>MSEFNITETYLRFLEEDTEMTMPIAAIEALVTLLRIKTPETAAEMINTIKSSTEELIKSIPNSVSLRAGCDIFMRFVLRNLHLYGDWENCKQHLIENGQLFVSRAKKSRNKIAEIGVDFIADDDIILVHGYSRAVFSLLNHAANKFIRFRCVVTESRPSKQGNQLYTLLEQKGIPVTLIVDSAVGAVIDKVDKVFVGAEGVAESGGIINLVGTYSVGVLAHNARKPFYVVTESHKFVRMFPLSSDDLPMAGPPLDFTRRTDDLEDALRGPTIDYTAQEYITALITDLGVLTPSAVSEELIKMWYD[2x];>MSESEAKSRSATPPSKAKQATPTTTAAANGEKKLTNKELKELKKQEKAAKRAAMKQANGISIEQQQQQAQMKKEKKQLQREQQQKREQKQKNANKKKQNERNVKKSTLFGHLETTEERRATILALTSAVSSPKTSRITAAGLMVPVVASALSGSNVLTASSLMPVGPNASSTVSASAPASTTTTLPASSAALSAGTSSASTNTPTAIQQEIASSNASDVAKTLASISLEAGEFNVIPGISSVIPTVLEQSFDNSSLISSVKELLLNKDLIHPSILLLTSHLAHYKIVGSIPRCIAMLEVFQIVIKDYQTPKGTTLSRNLTSYLSHQIDLLKKARPLSVTMGNAIRWLKQEISLIDPSTPDKAAKKDLCEKIGQFAKEKIELADQLIIDNASTQIEESTTIVTYGSSKVLTELLLHNAISLKKNIKVIVVDSRPLFEGRKMAETLRNAGVNVMYALITSLDTIFNMDVDYVFLGAHSILSNGFLYSRAGTAMLAMSAKRRNIPVLVCCESLKFSQRVQLDSVTFNELADPNDLVNIDYENPVERRGNKGALLNQFIKERKFEKKKLAMENKPKGNKIGGKKGSEGESKDASNEEDSNSKNILDGWQELPSLNIVNILYDLTPPEYIKKVITEFGALPPSSVPVILREYKGSA[2x];>[2x]MSSQAFTSVHPNAATSDVNVTIDTFVAKLKRRQVQGSYAIALETLQLLMRFISAARWNHVNDLIEQIRDLGNSLEKAHPTAFSCGNVIRRILAVLRDEVEEDTMSTTVTSTSVAEPLISSMFNLLQKPEQPHQNRKNSSGSSSMKTKTDYRQVAIQGIKDLIDEIKNIDEGIQQIAIDLIHDHEILLTPTPDSKTVLKFLITARERSNRTFTVLVTEGFPNNTKNAHEFAKKLAQHNIETLVVPDSAVFALMSRVGKVIIGTKAVFVNGGTISSNSGVSSVCECAREFRTPVFAVAGLYKLSPLYPFDVEKFVEFGGSQRILPRMDPRKRLDTVNQITDYVPPENIDIYITNVGGFNPSFIYRIAWDNYKQIDVHLDKNKA;>MAGKKGQKKSGLGNHGKNSDMDVEDRLQAVVLTDSYETRFMPLTAVKPRCLLPLANVPLIEYTLEFLAKAGVHEVFLICSSHANQINDYIENSKWNLPWSPFKITTIMSPEARCTGDVMRDLDNRGIITGDFILVSGDVLTNIDFSKMLEFHKKMHLQDKDHISTMCLSKASTYPKTRTIEPAAFVLDKSTSRCIYYQDLPLPSSREKTSIQIDPELLDNVDEFVIRNDLIDCRIDICTSHVPLIFQENFDYQSLRTDFVKGVISSDILGKHIYAYLTDEYAVRVESWQTYDTISQDFLGRWCYPLVLDSNIQDDQTYSYESRHIYKEKDVVLAQSCKIGKCTAIGSGTKIGEGTKIENSVIGRNCQIGENIRIKNSFIWDDCIIGNNSIIDHSLIASNATLGSNVRLNDGCIIGFNVKIDDNMDLDRNTKISASPLKNAGSRMYDNESNEQFDQDLDDQTLAVSIVGDKGVGYIYESEVSDDEDSSTEACKEINTLSNQLDELYLSDDSISSATKKTKKRRTMSVNSIYTDREEIDSEFEDEDFEKEGIATVERAMENNHDLDTALLELNTLRMSMNVTYHEVRIATITALLRRVYHFIATQTLGPKDAVVKVFNQWGLLFKRQAFDEEEYIDLMNIIMEKIVEQSFDKPDLILFSALVSLYDNDIIEEDVIYKWWDNVSTDPRYDEVKKLTVKWVEWLQNADEESSSEEE[2x];>[2x]MSIQAFVFCGKGSNLAPFTQPDFPFQTQNKDSTAATSGDKLNELVNSALDSTVINEFMQHSTRLPKALLPIGNRPMIEYVLDWCDQADFKEISVVAPVDEIELIESGLTSFLSLRKQQFELIYKALSNSNHSHHLQDPKKINFIPSKANSTGESLQKELLPRINGDFVILPCDFVTDIPPQVLVDQFRNRDDNNLAMTIYYKNSLDSSIDKKQQQKQKQQQFFTVYSENEDSERQPILLDVYSQRDVTKTKYLQIRSHLLWNYPNLTVSTKLLNSFIYFCSFELCQLLKLGPQSMSRQASFKDPFTGNQQQQNPPTTDDDEDRNHDDDDDYKPSATSIQPTYFKKKNDLILDPINCNKSLSKVFRDLSRRSWQHSKPREPIGIFILPNETLFIRANNLNAYMDANRFVLKIKSQTMFTKNIQIQSAAIGADAIVDPKCQISAHSNVKMSVLGTQANIGSRCRVAGSLLFPGVHLGDEVILENCIIGPMAKIGSKCKLSNCYIEGHYVVEPKNNFKGETLANVYLDEDEEDELIYDDSVIAGESEIAEETDSDDRSDEDSDDSEYTDEYEYEDDGLFER;>MSTSHCRFYENKYPEIDDIVMVNVQQIAEMGAYVKLLEYDNIEGMILLSELSRRRIRSIQKLIRVGKNDVAVVLRVDKEKGYIDLSKRRVSSEDIIKCEEKYQKSKTVHSILRYCAEKFQIPLEELYKTIAWPLSRKFGHAYEAFKLSIIDETVWEGIEPPSKDVLDELKNYISKRLTPQAVKIRADVEVSCFSYEGIDAIKDALKSAEDMSTEQMQVKVKLVAAPLYVLTTQALDKQKGIEQLESAIEKITEVITKYGGVCNITMPPKAVTATEDAELQALLESKELDNRSDSEDDEDESDDE[2x];>[2x]MSSDLAAELGFDPALKKKKKTKKVIPDDFDAAVNGKENGSGDDLFAGLKKKKKKSKSVSADAEAEKEPTDDIAEALGELSLKKKKKKTKDSSVDAFEKELAKAGLDNVDAESKEGTPSANSSIQQEVGLPYSELLSRFFNILRTNNPELAGDRSGPKFRIPPPVCLRDGKKTIFSNIQDIAEKLHRSPEHLIQYLFAELGTSGSVDGQKRLVIKGKFQSKQMENVLRRYILEYVTCKTCKSINTELKREQSNRLFFMVCKSCGSTRSVSSIKTGFQATVGKRRRM;>[2x]MSDLQDQEPSIIINGNLEPVGEPDIVEETEVVAQETQETQDADKPKKKVAFTGLEEDGETEEEKRKREFEEGGGLPEQPLNPDFSKLNPLSAEIINRQATINIGTIGHVAHGKSTVVRAISGVQTVRFKDELERNITIKLGYANAKIYKCQEPTCPEPDCYRSFKSDKEISPKCQRPGCPGRYKLVRHVSFVDCPGHDILMSTMLSGA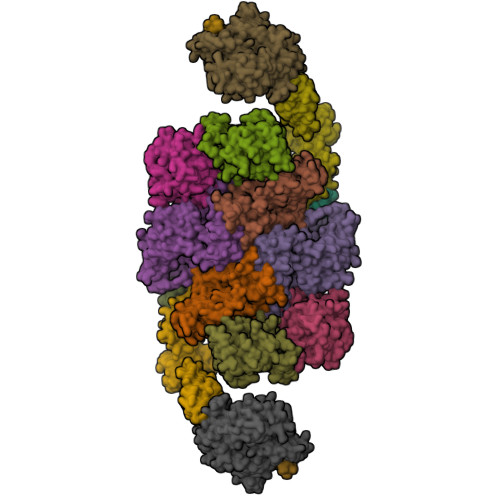AVMDAALLLIAGNESCPQPQTSEHLAAIEIMKLKHVIILQNKVDLMREESALEHQKSILKFIRGTIADGAPIVPISAQLKYNIDAVNEFIVKTIPVPPRDFMISPRLIVIRSFDVNKPGAEIEDLKGGVAGGSILNGVFKLGDEIEIRPGIVTKDDKGKIQCKPIFSNIVSLFAEQNDLKFAVPGGLIGVGTKVDPTLCRADRLVGQVVGAKGHLPNIYTDIEINYFLLRRLLGVKTDGQKQAKVRKLEPNEVLMVNIGSTATGARVVAVKADMARLQLTSPACTEINEKIALSRRIEKHWRLIGWATIKKGTTLEPIA In this work, we exhaustively probe the ability of all 36 immobile HJ sequences to form DNA crystals in two different designed systems. Three separate self-assembling DNA crystal systems are described in this report: the “4 × 5” and “4 × 6” designs (collectively referred to as the 4 × N systems), and a third construct with a “scrambled” sequence variant of the 4 × 6 lattices. Self-assembly was mediated by three constituent oligonucleotides: (S1) containing four sequence repeats of either 5 or 6 bases; (S2) composed of 21 bases containing complementary regions to both (S1); and (S3) which forms the second junction crossover. The HJ serves as the fundamental component at the core of each unit, and the ultimate assembly of the full lattice is facilitated by the complementary 2-base sticky ends that tail each duplex.

Each asymmetric unit could be defined as either a HJ containing 10 and 11 bp on each arm, or as a 21-bp linear duplex. The 4 × 5 system robustly crystallized with 75% of the junctions, and we obtained crystals in all but 9 of 36 sequences. In the 4 × 5 system, J25 and J34, both displaying P32 symmetry, crystallized in 50 mM Tris pH = 8.0 buffer containing cobalt hexamine (CoH18N6) and 10 mM MgCl2, and 50 mM HEPES pH = 7.5 with 20 mM MgCl2, respectively. Only cobalt could account for the different peaks in the Fo–Fc maps in J25, whereas in J34, and J22 and J23 in the 4 × 6 and 4 × 6 scramble systems, respectively, contained Mg2+. The modeled ions were readily superimposable, and well-coordinated at Pos1 & 2. To our knowledge, all experimental structures of HJs in the PDB database reported by diverse independent groups suggest that cations (e.g., Na+, Mg2+, Sr2+, Ba2+) should bind at this location. Of the resulting structures, 18 exhibited P32 symmetry with average cell dimensions a = b = 68.85 Å c = 60.09 Å, with only nine retaining the original P3221 symmetry with average cell edges a = b = 68.17 Å c = 60.60 Å. Although the cell parameters between the two symmetries were virtually indistinguishable, the differences between the periodicity of the lattices is dramatic, with vastly different cavity sizes. The P32 channels were treated as a hexagonal prism with 6.4 nm along each edge and a height measured from the top to the bottom of each block along with the average c-axis = 6.0 nm, with a resulting volume of ~639 nm3, a nearly 27-fold increase in cavity size relative to the P3221 lattices.

> GAGCAGACAAGACTCCACTCA;> AGTCT;> TCTGAGTGG;> TGTCTGC>ASLAADTPTACCFSYT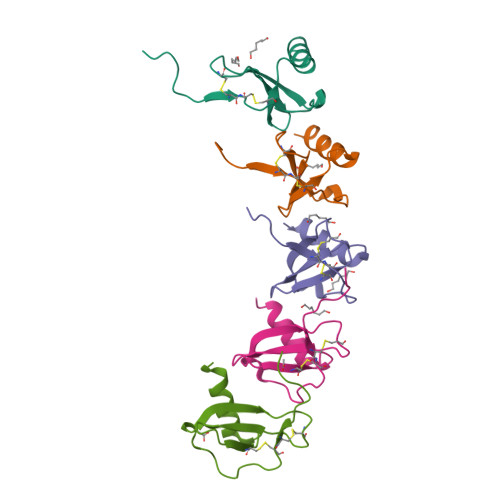SRQIPQNFIADYFETSSQCSKPGVIFLTKRSRQVCADPSEEWVQKYVSDLELSA[10x]N-(QUINOLIN-8-YL)METHANESULFONAMIDE | C10 H10 N2 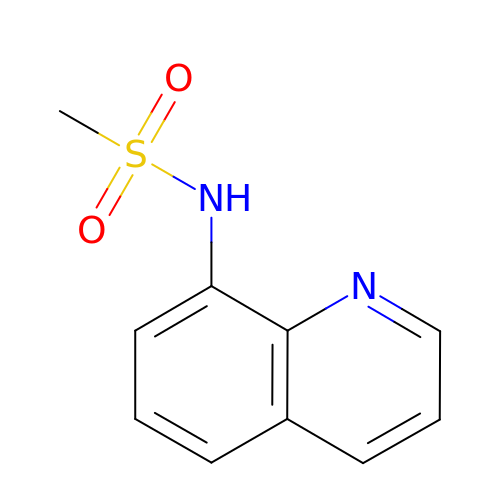O2 S | XYEPUTZVZYUENX-UHFFFAOYSA-N conserved and function as secondary active transporters. transport proteins that include the amino acid transporter LeuT18. μM range and that metal ion transport is coupled to the cotransport of protons. of the prokaryotic SLC11 transporter EcoDMT.

at a resolution of 3.3 Å. intertwined and aligned in opposite orientation within the membrane. that, in this crystal form, EcoDMT exhibits substantial structural differences. similarity to ScaDMT allows for a reliable comparison of equivalent segments. ScaDMT adopting an inward-facing and EcoDMT an outward-facing state. EcoDMT has now revealed the opposite endpoint within the transport cycle. equivalence of EcoDMT to an outward-facing state. α-helix 4 that is not observed in LeuT. be suitable for the coordination of Ca2+.

> MSETQSQTMTRPQDLSLSDINSTVEVPEGHSFWKTLLAYSGPGALVAVGYMDPGNWSTSITGGQNFQYLLLSIIVISSLLAMLLQNMAAKLGIVCQLDLAQAIRARTSRRLGFIFWILTELAIMATDIAEVIGAAIALYLLFKIPIFLAVVITVLDVFLLLLLNRIGFRKIEALVVCLIFVILFVFLYQIILSQPAWHQVAKGLIPSWASVQTSPKIGGQTPLSASLGIIGATIMPHNLFLHSAISQSRKIDRTDSSKVAEAVRFSNWDSNIQLSLAMVVNALLLIMGVAVFKSGAVQDPSFFGLYQALSNPDMVSNPVLAEAARSGVLSTLFAVALLASGQNSTITGTITGQVIMEGFIHLRLPLWLRRLVTRLIAIIPVVVCVAITSHQGSLDEHQALNNLMNNSQVFLALALPFSIVPLLMLTDSAAQMGNQFKNTRWVKVMGWLTVIILTLLNLISISSQIAGFFGDNPSSQDLLLSQVISIGIILAMIGLLIWTIIDIRRFTHPKQKALEVLFQ>[2x]MYKEPFGVKVDFETGIIEGAKKSVRRLSDMEGYFVDERAWKELVEKEDPVVYEVYAVEQEEKEGDLNFATTVLY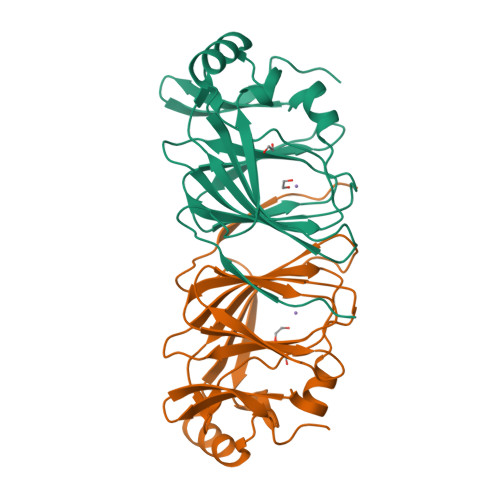PGKVGKEFFFTKGHFHAKLDRAEVYVALKGKGGMLLQTPEGDAKWISMEPGTVVYVPRGWAHRTVNIGDEPFIFLAIYPADAGHDYGTIAEKGFSKIVIEENGEVKVVDNPRWKK> EEIIWESLSVDVGSQGNPGIV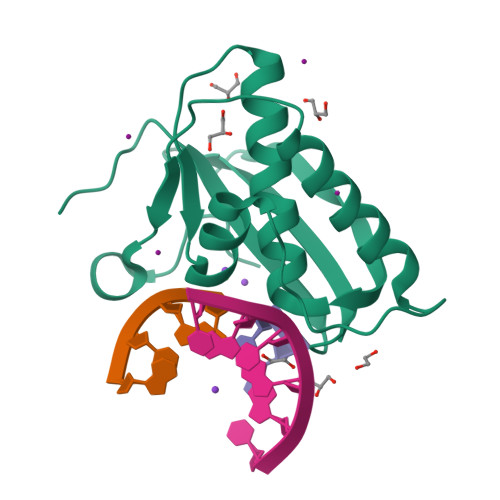EYKGVDTKTGEVLFEREPIPIGTNNMGEFLAIVHGLRYLKERNSRKPIYSDSQTAIKWVKDKKAKSTLVRNEETALIWKLVDEAEEWLNTHTYETPILKWQTDKWGEIKADY>[2x]MGSLTEDGLSYKEKFVVRSYEVGSNKTATVETIANLLQEVGCNHAQSVGFSTDGFATTTTMRKLHLIWVTARMHIEIYKYPAWGDVVEIETWCQSEGRIGTRRDWILKDSVTGEVTGRATSKWVMMNQDTRRLQKVSDDVRDEYLVFCPQEPRLAFPEENNRSLKKI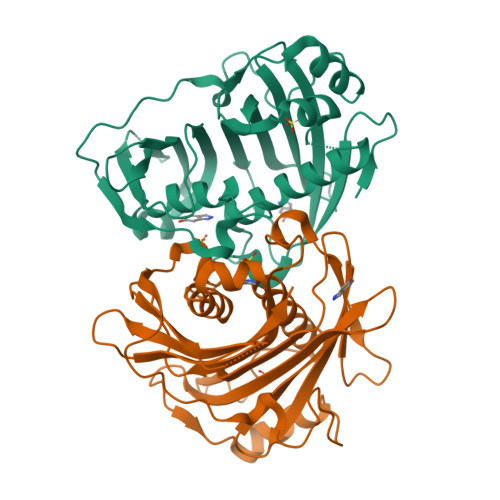PKLEDPAQYSMIGLKPRRADLDMNQHVNNVTYIGWVLESIPQEIVDTHELQVITLDYRRECQQDDVVDSLTTTTSEIGGTNGSATSGTQGHNDSQFLHLLRLSGDGQEINRGTTLWRKKPSSHHHHHH> MFVKLKGDLNGDGVINMADVMILAQSFGKAIGNPG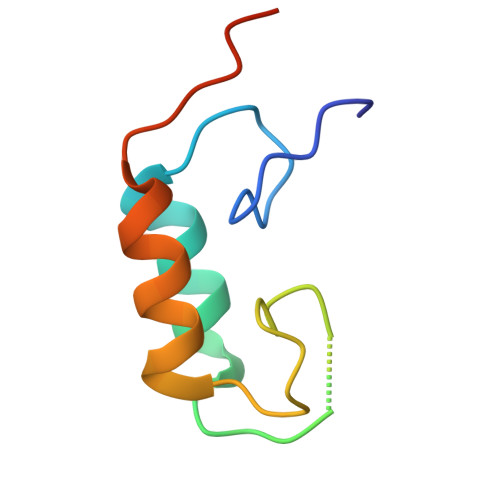VNEKADLNNDGVINSDDAIILAQYFGKTKSAEVVMF The 8.8a-oleandolide epoxygenase OleP, from Streptomyces antibioticus, is the P450 involved in the polyketide biosynthesis of the antibiotic oleandomycin. It introduces an epoxide function to the C8-C8a of the macrolactone ring of two structurally different intermediates, namely the aglycone 8.8a-oleandolide (DEO) and the C3-mono-glycosylated L-olivosyl-8.8a-deoxyoleandolide (L-O-DEO). Substrate binding to the cytochrome P450 OleP is coupled to a large open-to-closed transition that remodels the active site, minimizing its exposure to the external solvent. When the aglycone substrate binds, a small empty cavity is formed between the I and G helices, the BC loop, and the substrate itself, where solvent molecules accumulate mediating substrate-enzyme interactions.

As predicted, the substitution of G92 with a tryptophan and S240 with a tyrosine resulted in filling the solvent cavity, which is occupied by the bulky aromatic sidechains. This reduces to some extent the volume of the active site in both mutants, which is ~606.7 Å3 in the wild type and ~582.5 and ~566.8 Å3 in G92W and S240Y, respectively. In G92W and S240Y mutants, the bulkier and more hydrophobic groups are located in the cavity, causing, respectively, the partial and the total displacement of the solvent molecules and resulting in the formation of direct interactions between the enzyme and the substrate. In G92W, the tryptophan adopts a double conformation in conjunction with E89. In G92W, we identified: (i) A T-stacking interaction between W92 and F84 (BC loop) and F296 (β-hairpin β3); (ii) an induced dipole-dipole type interaction between the aromatic ring of W92 and the δ-carbonyl group of N236 and the ε-amino group of Q193. The G92W mutation is also able to alter the arrangement of the substrate with respect to the heme iron. The local analysis of the protein cavities as obtained by MD simulations show that in the G92W mutant the distance distribution maximum between the heme-iron and substrate is slightly higher than the WT and E89Y mutant. This might justify the uncomplete shift towards the high-spin state of the G92W mutant observed by means of UV-visible spectroscopy. Since the magnitude of the motions experienced by the BC loop (aa 83–100) in the open-to-closed transition is small (~3 Å), it is plausible that direct contacts of W92 with the substrate and the protein may be already formed in the open state.

>HMTDTHTGPTPADAVPAYPFSLPHALDLDPHYAELRRDEPVSRVRLPYGEGTAWLVTRMSDARIVLGDSRFSTAAATDPATPRMFPTPPEPDWVLAQDPPDHTRLRRLVGKAFTARRVEEMRPRVRSLVDSLLDDMVAHGSPADLVEFLAVPFPVAVICELLGVPLEDRDLFRTFSDAMLSSTRLTAAEIQRVQQDFMVYMDGLVAQRRDAPTEDLLGALALATDNDDHLTKGEIVNMGVSLLIAGHETSVNQITNLVHLLLTERKRYESLVADPALVPAAVEEMLRYTPLVSAGSFVRVATEDVELSTVTVRAGEPCVVHFASANRDEEVFDHADELDFHRERNPHIAFGHGAHHCIGAQLGRLELQEALSALVRRFPTLDLAEPVAGLKWKQGMLIRGLERQIVSW[6x]InlB is a surface-associated or secreted protein that mediates uptake of the pathogen Listeria monocytogenes into normally non-phagocytic cells by specifically stimulating the receptor tyrosine kinase MET on host cells. InlB consists of an internalin domain, a B-repeat and three GW domains. The internalin domain can be subdivided into an N-terminal helical cap domain, a leucine-rich repeat domain and an immunoglobulin-like inter-repeat (IR) domain. Using this approach the biochemical properties of the cap + LRR fragment, the IR domain, the B-repeat, the GW1 module and the GW2 + GW3 pair were addressed. These experiments showed that a cap + LRR fragment is sufficient for MET binding, but that the IR domain also contacts the receptor and contributes to MET activation.

To address a potential interaction of the InlB cap domain with a binding partner from the host cell, we sought to replace the cap by a structurally unrelated domain that still initiates folding. The hybrid protein combines residues 34–87 of YopM with residues 93–321 of InlB and will be referred to as YopM-InlB. The structure of YopM-InlB at 1.5 Å resolution confirms that this designed chimeric protein is properly folded. With a melting temperature (TM) of 49,9°C (+/−0.22°C) YopM-InlB was destabilized by about 2 K with respect to InlB321 containing the native N-terminal cap (TM of 51,9°C (+/− 0.21°C)). There are major shifts between wild type InlB and the hybrid protein in residues on the concave face of LRR1. The side chains of InlB Gln80 and Asn84 form hydrogen bonds to Thr646 and His644 of MET, respectively, in the crystal structure of the InlB:MET complex. Due to their relative shift, the equivalent atoms in the corresponding residues in YopM-InlB would no longer be able to form these hydrogen bonds. Instead rearrangements extend to LRR2 and to a lesser extent to LRR3. We had not anticipated this medium range effect, which can in retrospect be explained by a slightly lower curvature in the N-terminal region of the protein due to the absence of a 310 helix in the first LRR of YopM. The reduced affinity of YopM-InlB for MET is presumably due to the exchange of the first LRR along with the cap domain resulting in spatial shifts of residues from LRR1, LRR2, and LRR3, whose side chains are involved in MET binding.

> GAMGKSKAEYYNAWSEWERNAPPGNGEQRGMAVSRLRDCLDRQAHELELNNLGLSSLPGIQYLPNVTKLFLNGNKLTDIKPLANLKNLGWLFLDENKVKDLSSLKDLKKLKSLSLEHNGISDINGLVHLPQLESLYLGNNKITDITVLSRLTKLDTLSLEDNQISDIVPLAGLTKLQNLYLSKNHISDLRALAGLKNLDVLELFSQECLNKPINHQSNLVVPNTVKNTDGSLVTPEIISDDGDYEKPNVKWHLPEFTNEVSFIFYQPVTIGKAKARFHGRVTQPLKE> HMASMTGGQQMGRMSHMRPAFGAAW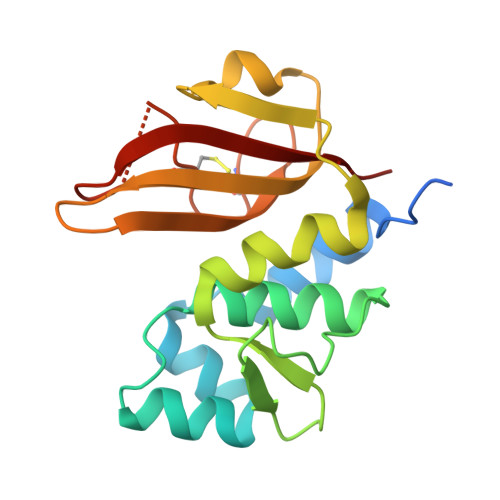NRFKEVNVNVEQVGKLLGGKVQHNIDAGIFKNACPIRMSYVLNYCGIPVPSNSKYATVTGSDKKRYMFRVKDMIAFLPTVLGKADISVSSPTPAQFAGKQGIIIFTGHGWLDATGHVTLWNGNICSDDCHFLGSPGNGSFIPTNATFWSLK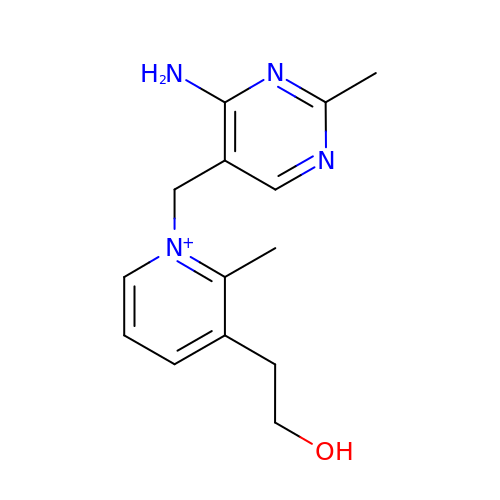1-[(4-AMINO-2-METHYLPYRIMIDIN-5-YL)METHYL]-3-(2-HYDROXYETHYL)-2-METHYLPYRIDINIUM | C14 H19 N4 O | PZWYDZMWPANLMB-UHFFFAOYSA-N We study the molecular properties of the membrane protein KtrAB—a member of the Trk/Ktr/HKT superfamily of transport proteins that shuffle K+ and Na+ ions across the plasma membrane, closely resemble K+ channels, and underlie environmental adaptation of cells of plants, fungi, bacteria, and archaea. KtrAB is formed by the KtrB membrane protein and the KtrA cytosolic ring protein. KtrB is responsible for ion permeation; each KtrB subunit has the architecture of a potassium channel pore domain, consisting of four M1-P-M2 (transmembrane helix 1-pore helix and loop- transmembrane helix 2) structural repeats (D1 to D4), which embrace an ion-permeable pore. KtrA binds to both ADP and ATP, resulting in a low-activity ADP-bound state and a high-activity ATP-bound state, respectively.

As an alternative, we turned to the KtrAΔCB complex, which is formed by wild-type KtrB and a C-terminal domain truncated form of KtrA (KtrAΔC). This KtrA form lacks residues 145 to 222 that correspond to the whole C-terminal domain. Thus, the stimulatory effect of ATP is abolished in KtrAΔCB, leading us to conclude that this complex is trapped in a low-activity state. As in the KtrAB-ATP and TrkHA structures, the asymmetric unit contains two membrane–protein dimers associated with opposing faces of an octameric RCK ring. Importantly, we could establish that KtrAΔCB-ADP and KtrAB-ADP are structurally similar and distinct from KtrAB-ATP. Importantly, the KtrAΔC ring is asymmetrically expanded along the diagonal defined by the tip contacts, revealing that in the KtrAB complex the ligand-dependent conformational change of the RCK ring occurs along the tip contacts. In the tip contact KtrA subunits, the Cα-Cα distance F71 distance increases from ~68 Å (KtrAB-ATP) to ~87 Å (KtrAΔCB-ADP), and for L66, from ~50 to ~76 Å. The position of the cytosolic end of the M1 transmembrane helix in repeat D2 (M1D2) in the averaged density is clearly different from the one seen in the KtrAB-ATP structure; the need for a positional adjustment of the helix is also detectable in a difference map. As a result of this conformational change, the M1D2 helix in KtrAΔCB-ADP has been straightened while in KtrAB-ATP it is bent towards the cytosolic pore. In addition, while all other KtrB helices are visible in the averaged electron-density map (including the pore helices and the M3 helices of repeats D2, D3, and D4), there is no density for the two helices just before M1D2, M3D1, and the D1-D2 loop helix; in KtrAB-ATP, these two helices, together with M1D2, form a domain-like structure (the D1-D2 domain) that functions as a KtrB foot on the tip contact.

>MGRIKNKQFAVIGLGRFGGSIVKELHRMGHEVLAVDINEEKVNAYASYATHAVIANATEENELLSLGIRNFEYVIVAIGANIQASTLTTLLLKELDIPNIWVKAQNYYHHKVLEKIGADRIIHPEKDMGVKIAQSLSDENVLNYLEGSKQFAVIGLGRFGGSIVKELHRMGHEVLAVDINEEKVNAYASYATHAVIANATEENELLSLGIRNFEYVIVAIGANIQASTLTTLLLKELDIPNIWVKAQNYYHHKVLEKIGADRIIHPEKDMGVKIAQSLSDENLELVPR[4x];>[4x]MTLQKDKVIKWVRFTPPQVLAIGFFLTIIIGAVLLMLPISTTKPLSWIDALFTAASATTVTGLAVVDTGTQFTVFGQTVIMGLIQIGGLGFMTFAVLIVMILAAAIGLKERMLVQEALNQPTIGGVIGLVKVLFLFSISIELIAALILSIRLVPQYGWSSGLFASLFHAISAFNNAGFSLWPDNLMSYVGDPTVNLVITFLFITGGIGFTVLFDVMKQRRFKTFSLHTALMLTGTLMLNAIAMLTVFILEYSNPGTLGHLAAVDKLWASYFQAVTPRTAGFNSLDFGSMREGTIVFTLLLMFIGAGSASTASGIKLTTFIVILTSVIAYLRGKKETVIFRRSIKYPIIIKALAVSVTSLFIVFLGIFALTITEQAPFLQIVFETFSAFGTVGLTMGLTPELTTAGKCIIIVIMFIGRIGPLTFVFSFAATEQSNIRYPDGEVFTG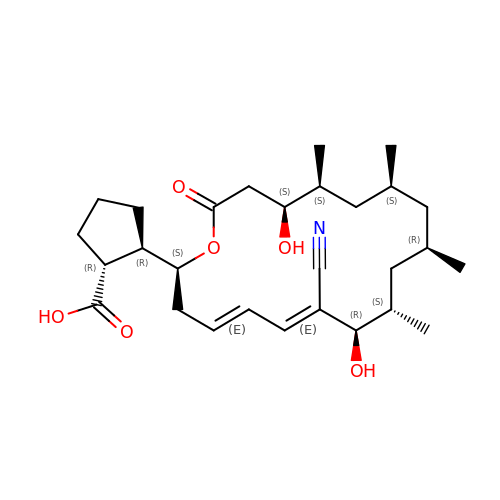(1R,2R)-2-[(2S,4E,6E,8R,9S,11R,13S,15S,16S)-7-cyano-8,16-dihydroxy-9,11,13,15-tetramethyl-18-oxooxacyclooctadeca-4,6-dien-2-yl]cyclopentanecarboxylic acid | C28 H43 N O6 | OJCKRNPLOZHAOU-RSXXJMTFSA-N> SSLPVPYKLPVSLSVGSCVIIK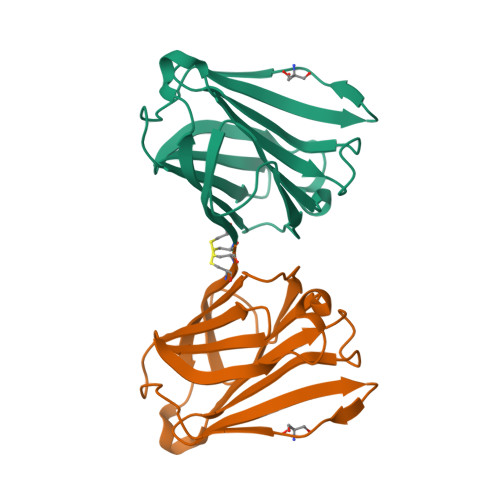GTPIHSFINDPQLQVDFYTDMDEDSDIAFHFNVHFGNHVVMNRREFGIWMLEETTDYVPFEDGKQFELCIYVHYNEYEIKVNGIRIYGFVHRIPPSFVKMVQVSRDISLTSVCVCN6-(2,4-dimethyl-1,3-thiazol-5-yl)-8-oxidanyl-3~{H}-quinazolin-4-one 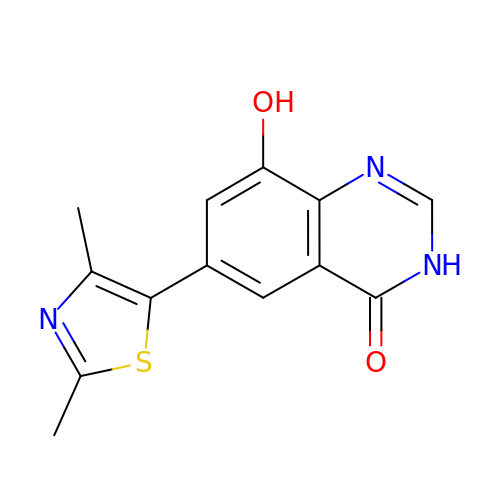| C13 H11 N3 O2 S | FCTDLOYVTPYHMT-UHFFFAOYSA-N>MGRENVLPVHNDVYEDFVFTTPYFQPESTFKSVPKLFSDILLGGVEWVYTTSESVLAYDYKLWYLWSGVSNLDESFDMFFNQYWALSLSTSVFQLFYAVILDRYLSVLFQNTPYTNDWFRMMLHSKETALIWLYHPELSWHINGLNQFFTYFYGGILEFVYFDKSNPDMCILVHTLWIHLLILFLIFTGFVTILFSFYGNPNTEENTIDSDYLAASGTVEAEKEITSIDDYLGLVFAIAYVFGVFFYVHGWTSMLSHAVLLLSCYSIIIMFLFILGMPTLLLYDFGIFFLAYLKGAGKYISSVAEMMFDYTACLVFYIRILAQWIRVVLMVVTFISLSHYVSDFDITNSALIGSENQSDSMNELNTNFSMTYYILTVLPGKFIYWIYEILHTFFVVCSQFVAFFAIVFWLFLFLYTFFIIEKHEDFFSKKREERKKKLKELWNLKN[2x];>MIRNFHSLVKRVPRLALTPFFGFRTSMTLADKKLSTGEASVVLAEKIKGITQQNDITEYGTVISIGDGIARVFGLTKVQAGEMVEFKSGIRGMALNLETDNVGVVVLGNDRDIKEGDVVKRTGAIVDVPIGEAMCGRVFDALGNPIDGLGPLKTTQRARVEIKAPGIIPRQSVRQPMQTGIKCVDSLVPIGRGQRELIIGDRQTGKTAIAIDTILNQKEAFNTGDVKKQLYCIYVAVGQKRSTIANLVSILKQHDCMKFTIVVCATASDAAPLQFLAPYSGCAIGEFFRDNGKHALIIYDDLSKQAVAYRQMSLLLRRPPGREAYPGDVFYLHSRLLERAAKMNDSLGGGSLTALPVIETQAGDVSAYIPTNVISITDGQIFLETELFYKGIRPAINVGLSVSRVGSAAQIKAMKKIAGNLKLTLATYRELAAFSQFGSDLDAKTQQQLNTGERLVEMLKQNQYTPMKVEEQVCIIFAGVKGFLDALVTSEVLKFEKKFLEHVRTNHSALLKRIRDSGDLSEVDTNELNTIIPLFIQEGGFKLKAQ[6x];>[2x]MHSTLRVFTKNNCLSFTNMNRFSTAAQVAQANYSKFRADYSASVAAFQQRIKTIEKENTGSMKKPMAKAYEHPYNSEHHPLNFSAVKIAETFHDFIGPEQVSPHYESFAMSRKFLLTFWGGFFVLNFGMATVDLNWIMKSTYIPWIFWFQLMYFYVEGKNSMFMPLLQRFYRRAAANEIFTMEAFYHENIENKLRNLMRITKGQLEYWDIHTSYGEIRADSINNFLANEYLRLQSHITSRALNILKQAQAYETMNQAALLQKLIDDATSAIDNALKGDKKAEVLARSLDSAIDGLSKGYMDYQNDPLLPLILSSIEANVKKITTLSAQEQANLIGLTAEQLKSIKENDVRARKEFLESQPKLDNNLKNIESVKKILATWGK;>[2x]MITILDYLFLLDLNDDLTRKAVFEQVIIFIFIYCTMNFLAWSTVVELIWPTHFFNRRHSSSQEFIRFRTYTEVLLKISAYNDFFYVLNNYYYNQKLILKN;>[2x]MSMLAKIAKNVVKTQALKNTTAAQTPSFQAPGNQDKILKWISTLSNKATTGESRSYCTQLSSLVSFYNKQHVEQIPTIDFNEWKSVISTQGLVDKVKENYESLIKEQYNTDAISKQISSASSKALDDIENELSFHAAIWLNAYADYTMFLFELEEYNDPNDYLMHENFDFFRGLETELEELTETHNYIPGAKDDVNLRGYLATQFAWGKKVISFYRHPADDFKCAKATKNMLGR;>[6x]MLSKALQRGIARAFSTTAKKEAPKTVKANGQVSQVIGAVVDVQFEGELPQILNALEVQGTQHRLVLEVAQHLGDSRVRTIAMDSTEGLVRGQPVVDTGLPISVPVGPGTLGRIMNVIGEPIDQRGPIKAAKLYPIHRDAPSFTDQATSAEILVTGIKVVDLLAPYARGGKIGLFGGAGVGKTVLIQELINNVAKHHGGYSVFAGVGERTREGNDLYHEMMDSKVISVKEGESRCALIFGQMNEPPGARARVGLTGLTVAEYFRDEEGKDVLLFVDNIFRFTQACSEVSALLGRIPSAVGYQPTLATDLGALQERITTTQKGSITSVQAIYVPADDLTDPAPATTFAHLDATTVLNRGLTELGIYPAVDPLDSTSRMLDPITIGEEHYTVARGVQKLLQDYKSLQDIIAILGVDDLSEEDKLVVARARKVQKFLSQPFFMSEVFSGIPGRFVNLKQNIASFKALLEGAGDEYPESCFYMKGDLEESLAAGRADALKSK;>[2x]MIHCLRNIRTVSALQSKISYNLGGGNKRKKTSGDLDNYDVLFVGANLGGICSNHFDKDTHGKYKCFVSFDQPINQIYSVRIPYEQQRVRKSEYIHFSKKSINQFTPSEMLAVKEILPEQNAVVLSSGRRIGYNQLVLATGLKHDFSQIKGFYEALEHPEHPVYANRDPETWRSAQHKYSKYISNFKSGDGYFCIPEYPYAGEVECFNFFVSDEVWKWAQHHGALSPKHTFTIVNANEKFVHYCDSADAFIKERLEKRGIRVEYNTKLLEVHQDGQKATFINTKTGEKSVRDYNNLYSIVPSKRQEFLDKAGLTNGNGLLNVDHQTLQHKKYKNIFGLGDAADLPTTKTFWAGWYQIAVVRNNVKRNLQGQTLNAHYDGFSKVPLFTGHQTLTYVAHSYGGVGNWQHLKHNNGGILAWMRYRSWAKGMAKKFQDFYNGARLGPPYHKVLKSFPELPGSPESQQSSGISKYFPTKTENKAAH;>MSLHEKMQTDYLWVKDHSQADSWAKARTHGYNYIAHTVPNKKERYEMIWRSMGKSTDWELEKFRLGKKFPDRGNKRRWFKNLFRLIKNPMGYIFWKTYKARLAKPSLIVTSMFIGFTLGFIKLKAQSIAYSKKQYATLRAGKNIEGSGQVHFGYHDQKWGMPAIPMFQLMYYELPGNSIVVNPCRNQNYRLYFEMRKKLGILPA[2x];>[2x]MINRSTAFISKNLRQANLTQSSLAMKTQYNQMGFSSDNPYNKRWEYKWKHSYYTYPRDYEHTEVRKPQDSKDVPPIYFAYYKDFVDRWLPGMNMWWQRRHRIFDKFNVYFLPGMSLFFYQFADLALGFKIMAAFPLFLAYTRIRDKTLDPDFKETYLRDMIYQNPEITKYFNEETIHVLDYEFEYLPGYLCPEKFPEYQNKTWQFFNTDTAQAEGFFKFGDVESGATMTLKFKTMPIPGKFRYQVGEPFYFYDLRAEIKCDGVYKEVVLVDEKESLKKIRPFLFLI;>[2x]MQVIRKHLAQKGLFNPFLFNRFSTQQDITSVPGDKPPAIEDSIHGKYAGVLFSSASSNKSLNKVAEDMKYFNQLYKESEVFKSFLNNVSLKRNQQRDIISALGKTNFNPATNNLLETLIENKRLDSLPKIAEKYMDYYRILNKQESITIISAQELTAAEKQKVEQGLKKGNANVQFTVVYQVDPAILGGLQMYSGNNFLDCSLLSRVNKLKTEIAKISF;>MQQRKKIYLRQKRKIYIQLKNKEKKKNNQFIQKREKMGYKIRNKSIFWTRAGWKNNWHPKNFNAPRPSYGEFTMGIRCRNDHHSFLRYVQTYRNMSRHCKQYFLGDKQLEETFILGLRSLFLVPYDSQCLTDQIKHGGERRFVDQLDRDFELISYNTHPYQLFTYTVRNEHLAWKNEQYEKIQKGEKTFEQELLDYLDEQVLAEKAKLRDGQNFSIERMTEIALHVFRKARAGKVRPAQDVRGPDGNVNDFLEQRRPFEHPNPTGVTH[2x];>[20x]MLLVKAVKVLVMGGCMLPIAFGALGTGVLFAGFNVALSRNPEETESLFNNTLMGFALIETFIFMSIGLGFFVLFAA;>MNPIQKAWLKILEPVSYVINEKMAKRTGIIGKLGRFFAIGPREYGVHPINRMFIFMNRKYMAFQAVALHRYSFVKSLTHNGFHMLRVFRHFAFVLPATVLAGLGLFVYWGDDNKCYSPDRFPYLKKRAGDMALPLNSLNQRTSAHYIEINAIYGAEMMKRYHKVWENIIEERSKATDQEKKTRYAHPSYQYSPLPVVSIPNVLNPLNLQ[2x];>[2x]MSENKAPGQIYAYDIHNTHYPYVNIKQDSQTQLLASFRRSIASINPFSYRQVPSQDRAAFGLRWGNAWYAPNPYPNGIHFDRVFPTHYDPLAETNRTKANLQLIKYAPGNYSTLVVTSEKLPRPCIRTIQNYRRCQMVNGTEKCNSEAQDILAICPNWALDHMKEKVRFYTKALAINNQTYIRAMQVEEYNQGRTVADVAPKTWIHGTRQHLRPDTMWADDRYTNITQTEINEAIKRVEARKAREHEKKPVEQANVNANTGEQPVRVEKSLYP;>[2x]MWYKYFSKQSWNLRVWRKANLKYNQDDFGMTQPKYIARFGDFRFRLVRTEGALRGCMFFVGFGCFSIINYLYGRYGYIINESSQKRAAQDLLDNDMAADKILFKNRVGAPTRPLRSLDDMMAFLSGSATYDQLADYASYNHAMDVNQDQQAGLDSWMSEKDKNMVKYYQRSLGKKVEGI;>[2x]MPVKEGQAKLWFSTKEEADAYDDKMISNIELKSQDYEDENFSPVFNRKTQEYFLEPSEKFKSDFAELLRPLRSLSFNQVVDRYVLIPPNHTFYRNWTYEKFLGGFGLSYLILRELPLRNFYARVFVMYAFAAKVLDHLGNPFPFSGHGQIVAAADRWNHWDVRCYDNVMKALKYIRIPTVQNNIPEATRWYGRQPGHLLRADTYWIPNLVSQRFAKHQPAHWDGTQNMPIFRLADPKHKDSYMVQFR;>[2x]MDNYFTAITLLGLRDQNLPPFKDARLQRYKSIKKMIDLIETTTKLAPPMPVELFMLNPTDPEWDDDMTYPTITHATALYKSSALAGNLFLYAYNYNNFTANIRLRTMRYLFPVVSLAIFGNIYWDYRSQLVKVNLFDEYIQARAQELVKQNEYLLEHEDVKRYVWWYEDLKETLARVHRQANNHKACDFKDSEIILQDFIRRYTNPKDNLPIKFHPQGQTF;>[2x]MEGFIQNKRKKEKEGEEEEESKEKRKQINQLNKQKQEEEKIYQQKKDQKRKKYLYQRKEMTIFAETWEASEYQYRNKANLKTLPVNHLGKLAELKFDFVEYKAHQLIACHLYERMTIHCMNQYGLFKDFYRPECLDAQYYFKTCVELNAAYGI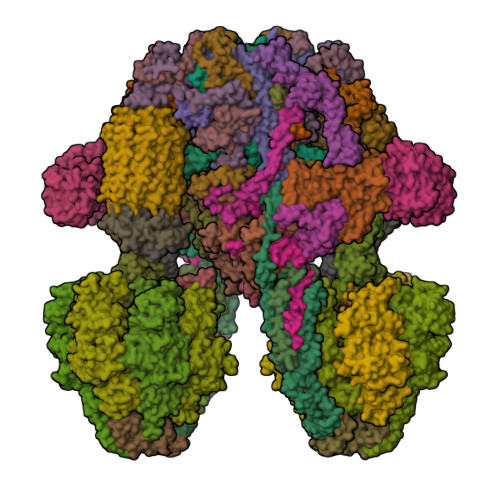QKKFFPEHFVGSPYARPVPQFQQLGL;>[2x]MKQKINKLLKNKGVQDKYKYLSKLILLDQEIKGKIKRKNKKEKQKRKNKLILEEMQNTTNIVHVPVHMGHTHYFDYIDSFPKLKEGPTLEENHITNQKILREQLISGQQGLEQNLCLRNCFKLSQKRYIEFCLDRKCGGADFQRAATILGYTKN;>MSNIFLELQDGDKTVYTHTSLIEESKQEQIQAIYDKVPQWTNGGRFLGFWLSMEAVNRVQSVAKLPIYYRAGIVATSTLLGGLVSSLVFWKSGNENQVAKLANGAPVYLKKWEVPELSKLYFFLDDDNNFKPSLNHHAVTQGRQYYKIYQHN[2x];>MFRNILSLVTKPSKLSQKTFYNFAAAKNEVQVSKKQQQAGAKRDLTQYVEGQIVNRNQLTLKKQEDIEQYVLKLVRGYFRTTNKQGLNINSVLQDHGLDEFDSIELAMQVEEDLGYVISAETIPVLNKVKHFVNYINHVEQFKAENGKAPIA[2x];>[2x]MSQDPKIVNPQLWPNPNKLRFADLYKYQGVEMKKINDSIKNYKAAKFYIGGILGGCLVFKFFIDAAVDKYIFGENGNGGKFLEMQTINSNYDYYYNRQFQRMRYLTEDPAGDDPLQKTKDEHLVDLGFIPKVFGANVEVRKRAPHDKYL;>MNSLSSKKANSLVFKSIRNFTLQWGSLAERPMVDRVMSTSTWPVPYYQRLFKAYPIREKKDKMSLLLSDIDIDDTNWYQAKDFLRGSFRGRQIVDYVENNIASNTYILIQQDVANMAKAYVHDICGYIDVANKENVRILSKGDLI[2x];>[2x]MFTRFVTQPTLLTQTQRALFSALTKKQKMEVTLRTPYKEYLANFDGFSRITAKTNEASLVIQNKTPASLYVLPPGPLKIRFTSEVKNVSGDFLHTGGWVIVHADNTCEINVMDLFDRKEVRADQFEKGNIQDLDTLAGKYAAKSRKSTVRLFTKATTQ;>[2x]MCIEFAFKKAGIPIVRNFLHSTEGVIYGLPQRVQRNLAINYTVKQYKEGKAVSAKTIKTLQEAFPSKGDTK;>[2x]MFGLASKGFINTSLVMVPQMNFGANLKQLKIRMKAIGSIKKITKAMKMVAASKMKAETSRLENGRNFAVGSVQKMLENESYVQKKKSTTAPKSTLLVPITSDKGLCGSVNSSIVREVKRLALNNRSAFGLLPVGEKGSSGLSRPFPDLLKSSIVNIQNVNFPTAAAIAHQVSTQGAGYDQVTLIYNHFKNAISYVVKHQELLPRAQFLNLFKYVTRHEAVEPELEYSKNYFFELYMASSVYNALLNSSASEQASRMNAMENASKNAGEILSKLTLDYNKARQAKITMELIEIISGASIV;>MNRSVNIAKNLIQTYRAMSVQSRFAFSTREEEWLDKRTKSQEKVYFDQEDRKAMKRLLEKLNTTSKFVEDSEYLAPQNLEVENILKRYHINYTQALIDELVDWKTGKN[2x];> MKMEYLQSEEKKDAINKQIHKKEEKEEKEIKIKRKNKVKQRIQIINQIKKYIEAKQQKKQIQSKNQRKYKGRMINTRKQVFKCLWGAQPAYNFSRIINHLRGDPVYQDNTKDVSLRGTFLRGKYDDLPTMIFFTEACDLTANWIPFFTNPQYDILAHRNVWLLNPRNFGNSDRHPSFDLQEMSDDVMRFMYSQKISMATLGGHGIGGKIALAVGCYHAERVTGVFSIDSSPMDQRYHEAFKEFKGYVNALTEINFKTWSDKDVKVFLKENIKDPKWRSIFTNNISKNAKTQSDSFNFEINYLNHNLNFNKADSLGNWAVKNGIYTGRAHFIFPEYSRWVHLATNTLPMHKVCARVKGFGHDIFYVQGDENPLNHWVYDFENYANVVASKLNKFLHSYDGVHALLKDRTEIGNFMIPDRIKSRNDSKHIYGDYSPAHLHHNWRFNHIYEKHDELDKKLNEQ> GP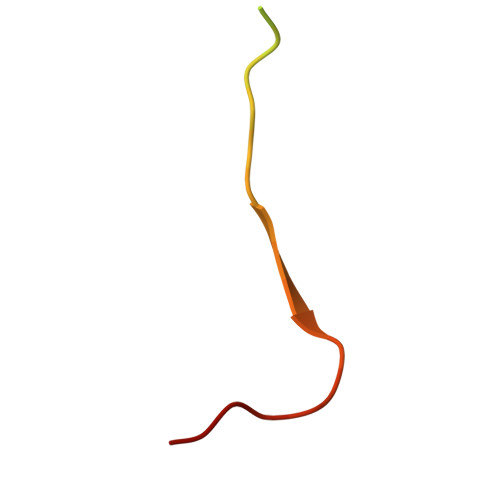GGSGSGGPCCSHARIPRTPYLVLSYVNGLPPV The zinc-dependent metalloprotease meprin α is predominantly expressed in the brush border membrane of proximal tubules in the kidney and enterocytes in the small intestine and colon. In normal tissue homeostasis meprin α performs key roles in inflammation, immunity, and extracellular matrix remodelling. In contrast to meprin β, meprin α is secreted into the extracellular space, whereupon it oligomerises to form giant assemblies and is the largest extracellular protease identified to date (~6 MDa). Here, using cryo-electron microscopy, we determine the high-resolution structure of the zymogen and mature form of meprin α, as well as the structure of the active form in complex with a prototype small molecule inhibitor and human fetuin-B. Our data reveal that meprin α forms a giant, flexible, left-handed helical assembly of roughly 22 nm in diameter.

Our data show that both the zymogen and active form of the meprin α ectodomain (i.e., the region released through furin cleavage) is capable of self-association to form a flexible, giant helical assembly. The zymogen form of meprin α is plugged by an α-helical pro-peptide that sterically occludes the active site. The pro-peptide forms a small helical cork which plugs the active core and thus sterically occludes the active site. Accordingly, the steric occlusion of the active site represents the major autoinhibitory mechanism. In a single asymmetric unit of the helix, two meprin α subunits homodimerise into a C2 arrangement via the M12A and MATH domains. The dimer interface is most extensive (1374 Å2) and highly conserved between both meprin α and meprin β. This interface is defined by the M12A protease and MAM domains, which are dependent on a conserved MAM/MAM disulphide bond to form the covalently linked homodimer. Two identical MAM/MATH interfaces (610 Å2) each provided by two homodimers together drive the head-to-tail formation of the non-covalent helical assembly of multiple homodimers. This latter interface is defined by extensive charge complementarity and salt bridges between the MAM and MATH domains and has a calculated cumulative solvation free energy (ΔiG) of −5.2 kcal mol−1. The MAM and MATH domains buttress the protease domain, forming the outer structure of the helix interacting via a head-to-tail arrangement, while at the dimer interface a conserved disulphide bond stabilises MAM/MAM interactions (see next section). This arrangement of dimers forms an indefinite filament which coils into a left-handed helical ultrastructure. Cleavage of an exposed flexible loop, defined by residues L61-L67 located distal to the active site, releases the pro-peptide and exposes the catalytic core of the active site.

>[4x]WSHPQFEKVPIKYLPEENVHDADFGEQKDISEINLAAGLDLFQGDILLQKSRNGLRDPNTRWTFPIPYILADNLGLNAKGAILYAFEMFRLKSCVDFKPYEGESSYIIFQQFDGCWSEVGDQHVGQNISIGQGCAYKAIIEHEILHALGFYHEQSRTDRDDYVNIWWDQILSGYQHNFDTYDDSLITDLNTPYDYESLMHYQPFSFNKNASVPTITAKIPEFNSIIGQRLDFSAIDLERLNRMYNCTTTHTLLDHCTFEKANICGMIQGTRDDTDWAHQDSAQAGEVDHTLLGQCTGAGYFMQFSTSSGSAEEAALLESRILYPKRKQQCLQFFYKMTGSPSDRLVVWVRRDDSTGNVRKLVKVQTFQGDDDHNWKIAHVVLKEEQKFRYLFQGTKGDPQNSTGGIYLDDITLTETPCPTGVWTVRNFSQVLENTSKGDKLQSPRFYNSEGYGFGVTLYPNSRESSGYLRLAFHVCSGENDAILEWPVENRQVIITILDQEPDVRNRMSSSMVFTTSKSHTSPAINDTVIWDRPSRVGTYHTDCNCFRSIDLGWSGFISHQMLKRRSFLKNDDLIIFVDFEDITHLS> MIKEMIEDFISKGGLIFTHSGRYTNTNNSCFIFNKNDIGVDTKVDMYTPKSAGIKNEEGENLWQVLNKANMFYRIYSGELGEELQYLLKSCCTAKEDVTTLPQIYFKNGEGYDILVPIGNAHNLISGT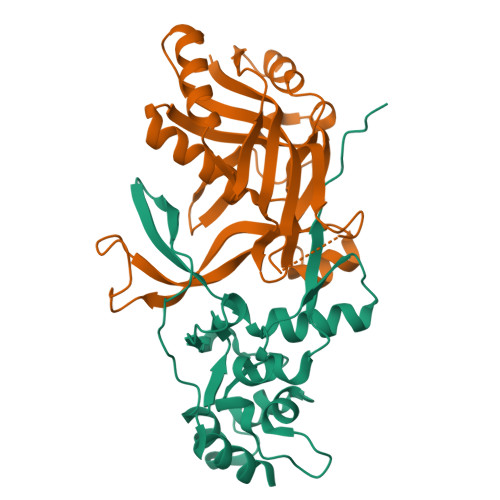EYLWEHKYYNTFTQKLGGSNPQNCTHACNKMRGGFKQFNCTPPQVEDNYNA;> MRKFIIVKNVKVDGINAKSSDITVGMPPATTFCGLGETMSIKTGIVVKAVSYGSVKFEVRGSRFNTSVTKFAWQDRGNGGKANNNSPIQPKPLADGVFTLCFEVEWEDCAEVLVDKVTNFINTARIAGGTIASFNKPFVKVAKDAEELASVKNAMMPCYVVVDCGVEVNIFEDAVNRKLQPMVNGYKKLEKIVDNKHMRDKFTPAYLATPTYTMIGYKMVSNVDNFDQALWQYGENTKVKTIGGIYND> IVGGQECKDGECPWQALLINEENEGFCGGTILSEFYILTAAHCLYQAKRFKVRVGDRNTEQEEGGEAVHEVEVVIKHNRFTKETYDFDIAVLRLKTPITFRMNVAPACLPERDWAESTLMTQKTGIVSGFGRTHEKGRQSTRLKMLEVPYVDRNSCKLSSSFIITQNMFCAGYDTKQEDACQGDSGGPHVTRFKDTYFVTGIVSWGEGCARKGKYGIYTKVTAFLKWIDRSM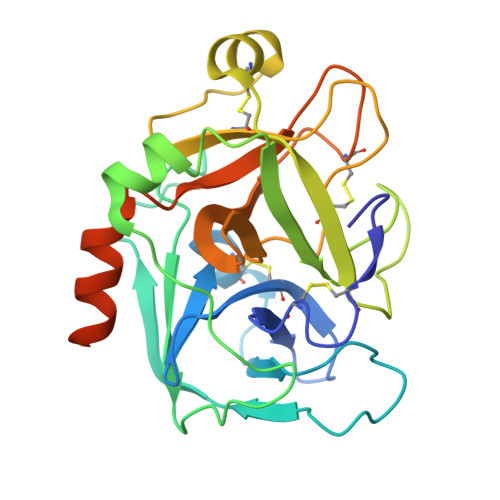KTRGLPKAKSHAPEVITSSPLK> MFAWWGRTVYQFRYIVIGVMVALCLGGGV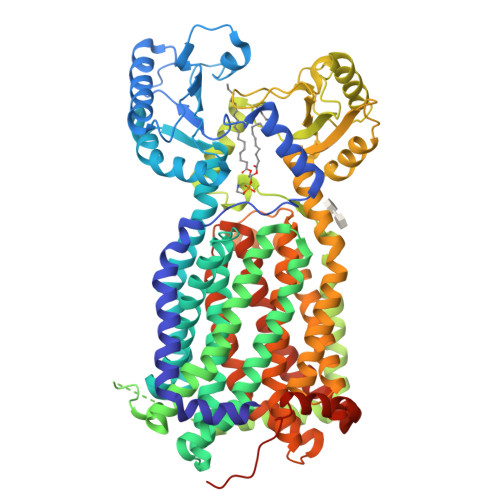YGISLGNHVTQSGFYDEGSQSVAASLIGDEVYGRDRTSHVVAILTPPDDKKVTDKAWQKKVTEELDQVVKDHEDQIVGWVGWLKAPDTTDPTVSAMKTQDLRHTFISIPLQGDDDDEILKNYQVVEPELQQVNGGDIRLAGLNPLASELTGTIGEDQKRAEVAAIPLVAVVLFFVFGTVIAAALPAIIGGLAIAGALGIMRLVAEFTPVHFFAQPVVTLIGLGIAIDYGLFIVSRFREEIAEGYDTEAAVRRTVMTSGRTVVFSAVIIVASSVPLLLFPQGFLKSITYAIIASVMLAAILSITVLAAALAILGPRVDALGVTTLLKIPFLANWQFSRRIIDWFAEKTQKTKTREEVERGFWGRLVNVVMKRPIAFAAPILVVMVLLIIPLGQLSLGGISEKYLPPDNAVRQSQEQFDKLFPGFRTEPLTLVMKREDGEPITDAQIADMRAKALTVSGFTDPDNDPEKMWKERPANDSGSKDPSVRVIQNGLENRNDAAKKIDELRALQPPHGIEVFVGGTPALEQDSIHSLFDKLPLMALILIVTTTVLMFLAFGSVVLPIKAALMSALTLGSTMGILTWMFVDGHGSGLMNYTPQPLMAPMIGLIIAVIWGLSTDYEVFLVSRMVEARERGMSTAEAIRIGTATTGRLITGAALILAVVAGAFVFSDLVMMKYLAFGLLIALLLDATIIRMFLVPAVMKLLGDDCWWAPRWMKRVQEKLGLGETELPDERKRPTVRESETDQRHHHHHH>PLLIFSGQSNRPLAQAIAEALGLPLGKSTTLRFANDNLFVRYEESLREGDVFIVQSFVPPVQDHLMELLMMVDAAKGASAARVTAVIPYFSYARSDKKDAPRISITARLIADLLQTAGADRVLTMTLHSPQVHGFFKIPVDHLSAEPVIANYF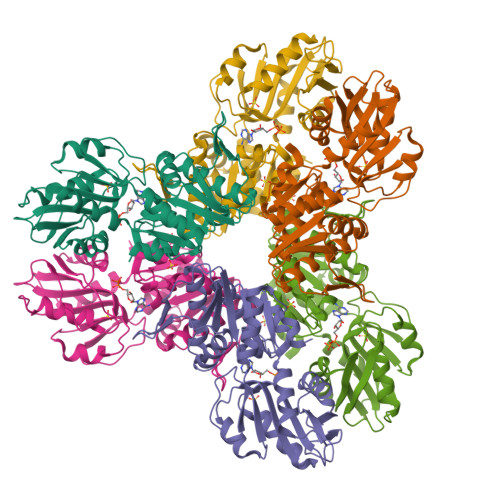ATRVDLENAVVVAPDAGDLKRASALARRLGLPLAFIDKERVSDTEVRVRMLVGEVEGKTALIVDDEISTAGSLVEAVEALMQAGAKEVYAAATHGVYVGPALDRIAKSPVKEVAATDTCPPKEGPKLRTLTVAPLFAEAIWRIHRGESVSSLFT[3x]3-[3-[3-[(4~{S})-6-azanyl-5-cyano-3-methyl-4-propan-2-yl-2~{H}-pyrano[2,3-c]pyrazol-4-yl]-5-fluoranyl-phenyl]phenyl]propanoic acid | C26 H25 F N4 O3 | 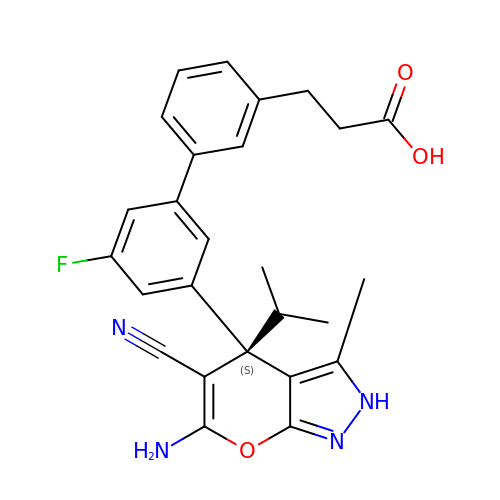MGFALDRJNSGSKD-SANMLTNESA-N>FNILLATDSYKVTHYKQYPPNTSKVYSYFECREKKTENSKLRKVKYEETVFYGLQYILNKYLKGKVVTKEKIQEAKDVYKEHFQDDVFNEKGWNYILEKYDGHLPIEIKAVPEGFVIPRGNVLFTVENTDPECYWLTNWIETILVQSWYPITVATNSREQKKILAKYLLETSGNLDGLEYKLHDFGYRGVSSQETAGIGASAHLVNFKGTDTVAGLALIKKYYGTKDPVPGYSVPAAEHSTITAWGKDHEKDAFEHIVTQFSSVPVSVVSDSYDIYNACEKIWGEDLRHLIVSRSTQAPLIIRPDSGNPLDTVLKVLEILGKKFPVTENSKGYKLLPPYLRVIQGDGVDINTLQEIVEGMKQKMWSIENIAFGSGGG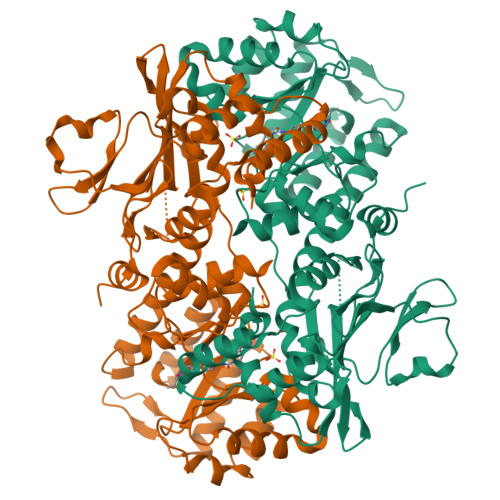LLQKLTRDLLNCSFKCSYVVTNGLGINVFKDPVADPNKRSKKGRLSLHRTPAGNFVTLEEGKGDLEEYGQDLLHTVFKNGKVTKSYSFDEIRKNAQLNIE[2x]> A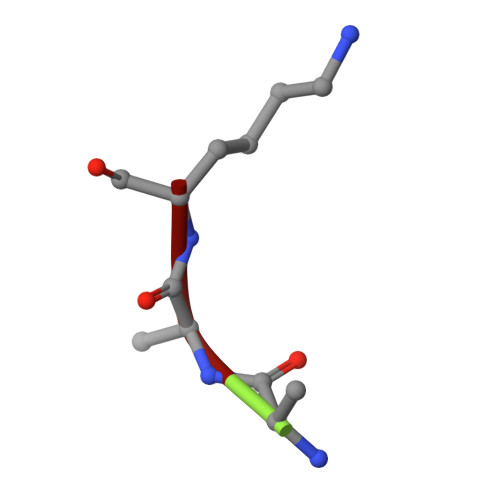AK>MTNEYVVTMSSLTEFNPNNARKSYLFDNYEVDPNYAFKAMVSFGLSNIPYAGGFLSTLWNIFWPNTPNEPDIENIWEQLRDRIQDLVDESIIDAINGILDSKIKETRDKIQDINETIENFGYAAAKDDYI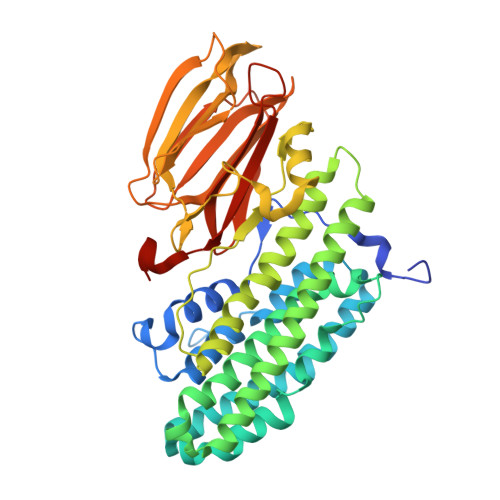GLVTHYLIGLEENFKRELDGDEWLGYAILPLLATTVSLQITYMACGLDYKDEFGFTDSDVHKLTRNIDKLYDDVSSYITELAAWADNDSYNNANQDNVYDEVMGARSWCTVHGFEHMLIWQKIKELKKVDVFVHSNLISYSPAVGFPSGNFNYIATGTEDEIPQPLKPNMFGERRNRIVKIESWNSIEIHYYNRVGRLKLTYENGEVVELGKAHKYDEHYQSIELNGAYIKYVDVIANGPEAIDRIVFHFSDDRTFVVGENSGKPSVRLQLEGHFICGMLADQEGSDKVAAFSVAYELFHPDEFGTEKLEHHHHHH[2x]DNA-stabilized silver nanoclusters (DNA-AgNCs) are emissive systems comprising a small aggregate of silver atoms and cations wrapped in one or multiple DNA strands. The Ag16NC is embedded in two 10-base oligomers (5′-CACCTAGCGA-3′), containing two guanosines. We therefore designed three inosine (I) mutants: I7 (5′-CACCTAICGA-3′) and I9 (5′-CACCTAGCIA-3′), where the guanosine in position 7 and 9 was replaced respectively, and I7–I9 (5′-CACCTAICIA-3′) where both guanosines were substituted. Single crystal X-ray diffraction measurements unravelled the structure of the I7 and I7–I9 mutants, allowing us to understand how the observed spectroscopic changes are related to the amino groups in position 7 and 9.

The G7 base in DNA-Ag16NC coordinates two silvers via N7 and O6, while the hydrogen atoms on N1 and N2 of G7 can form hydrogen bonds with O2 of T5 (2.8–3.1 Å). The I7 mutant lacks the N2 amino group and the increased distance between N1 of I7 and O2 of T5 indicates that no hydrogen bonds can be formed. Intriguingly, the deprotonated N1 of one of the I7 bases is coordinated by Ag with an occupancy of 0.57. This is most likely a silver cation, which interacts at the same time with the oxygen of a water molecule (not shown). Emission spectra and decay times of the crystals confirm that the crystal structure is a good proxy for the solution structure. When position 7 was replaced, the absence of the amino groups resulted in the lack of hydrogen bonds with T5, which made the construct less rigid. This could be the reason for the shortening of <τw> and the decrease of Q by increased contribution from vibration-mediated non-radiative decay pathways. Our results indicate that, while the base in position 5 was not directly bound to the AgNC, the hydrogen bonding interactions with it have an important role for the overall flexibility of the construct. Interestingly, the microsecond luminescence decay time <τμs> is lower for the I7 and I7–I9 mutants, while it is unaffected for the I9 modification, indicating that position 7 plays a more relevant role for <τμs>.

>[2x]CACCTAICGA>[2x]SMPRVDFPRSRLRFKEKLGEGQFGEVHLCEVDSPQDLVSL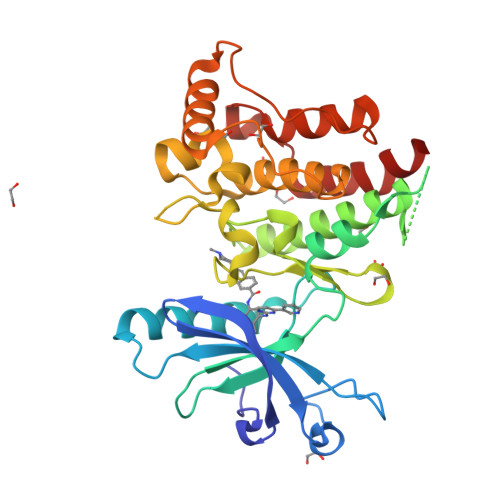DFPLNVRKGHPLLVAVKILRPDATKNARNDFLKEVKIMSRLKDPNIIRLLGVCVQDDPLCMITDYMENGDLNQFLSAHQLEDKAAEGAPGDGQAAQGPTISYPMLLHVAAQIASGMRYLATLNFVHRDLATRNCLVGENFTIKIADFGMSRNLYAGDYYRVQGRAVLPIRWMAWECILMGKFTTASDVWAFGVTLWEVLMLCRAQPFGQLTDEQVIENAGEFFRDQGRQVYLSRPPACPQGLYELMLRCWSRESEQRPPFSQLHRFLAEDALNTV Doublecortin-like kinase 1 (DCLK1) is a multi-domain bi-functional protein that belongs to the protein kinase superfamily and the doublecortin (DCX) family within the microtubule-associated protein (MAP) superfamily. Doublecortin-like kinase 1 (DCLK1) is an understudied bi-functional kinase with a proven role in tumour growth and development. Multiple isoforms of DCLK1 exist, generated by alternative splicing. Here, we report the crystal structures of DCLK1 kinase domain in complex with DCLK1-IN-1 and its precursors.

To further probe the R4 position, an electronegative trifluoroethyl group was introduced instead of hydrophobic ethyl, which led to DCLK1-IN-137. To better understand the effect of this change, we crystallised DCLK1-KD in complex with DCLK1-IN-1 to 3.1 Å resolution. However, a striking feature of the DCLK1-KD:DCLK1-IN-1 structure, is an opening of the ATP binding site to accommodate the bulkier trifluoroethyl group. The specific orientation adopted by the trifluoroethyl group allows additional contacts with residues Val404, Ala417 and Met465. In addition, the N-lobe undergoes a twist that shifts the positions of the β strands between 2.5 and 3.5 Å. The region near the glycine loop also undergoes an upward shift by 5 Å (distance measured at the position of Cα of Ile396 located at the start of the glycine loop and Ala402 located at the end of the loop). Notably, the presence of the trifluoroethyl group disrupts the salt-bridge interaction between the β3 strand invariant lysine (Lys419) and the conserved the αC helix glutamate (Glu436). Interestingly, this opening creates a shallow pocket, which in our structure is occupied by an additional electron density seen in both copies of DCLK1 that could be attributed to a fragment of polyethylene glycol (PEG), a component of the crystallisation condition. Overall, these changes can account for the dramatically increased DCLK1-IN-1 selectivity for DCLK1 against ERK5, LRRK2 and BRD428 and raise the possibility that the space occupied by the PEG molecule could be further explored for the design of DCLK1 selective inhibitors.

>GSGEEVSEEGFQIPATITERYKVGRTIGDGNFAVVKECVERSTAREYALKIIKKSKCRGKEHMIQNEVSILRRVKHPNIVLLIEEMDVPTELYLVMELVKGGDLFDAITSTNKYTERDASGMLYNLASAIKYLHSLNIVHRDIKPENLLVYEHQDGSKSLKLGDFGLATIVDGPLYTVCGTPTYVAPEIIAETGYGLKVDIWAAGVITYILLCGFPPFRGSGDDQEVLFDQILMGQVDFPSPYWDNVSDSAKELITMMLLVDVDQRFSAVQVLEHPWVND[2x]>[2x]MELEDANVTKKVELRPLIGLTRGLPPTDLE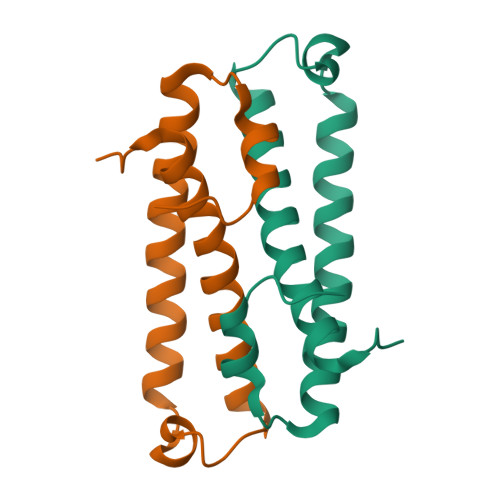TITIDAIRTHRRLVEKADELFQALPETYKTGQACGGPQHIRYIEASIEMHAQMSALNTLISILGFIPKVVVN1S-8AB-OCTAHYDRO-INDOLIZIDINE-1A,2A,8B-TRIOL 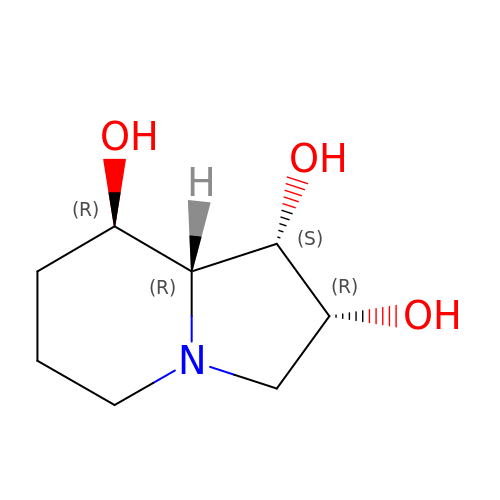| C8 H15 N O3 | FXUAIOOAOAVCGD-WCTZXXKLSA-N> AGSGHMMELHILEHRVRVLSVARPGLWLYTHPLIKLLFLPRRSRCKFFSLTETPEDYTLMVDEEGFKELPPSEFLQVAEATWLVLNVSSHSGAAVQAAGVTKIARSVIAPLAEHHVSVLMLSTYQTDFILVREQDLSVVIHTLAQEFDIYREVGGEPVPVTRDDSSNGFPRTQHGPSPTVHPIQSPQNRFCVLTLDPETLPAIATTLIDVLFYSHSTPKEAASSSPEPSSITFFAFSLIEGYISIVMDAETQKKFPSDLLLTSSSGELWRM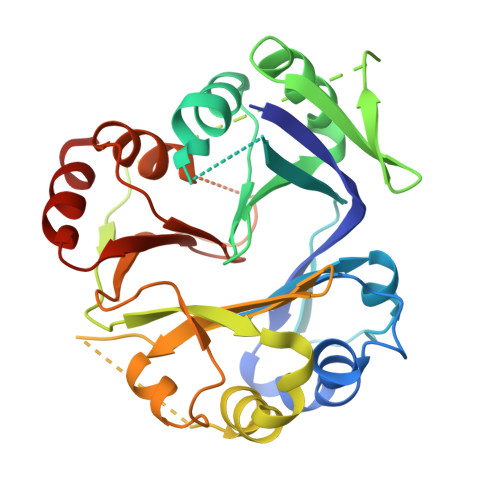VRIGGQPLGFDECGIVAQIAGPLAAADISAYYISTFNFDHALVPEDGIGSVIEVLQRRQEGLAS To address this problem, we investigated a cross-seeding approach with a mixture integrating a heterogeneous set of protein crystal fragments to be used as generic seeds. The fragments are nanometre-sized templates chosen to promote crystal nucleation of protein samples unrelated to the proteins forming the seeds. To demonstrate applicability, the generic cross-seeding mixture was simply added to a sample of the human retinoblastoma binding protein 9 (RBBP9) before proceeding with crystallization.

An atypical crystal form of the human serine hydrolase retinoblastoma binding protein 9 was obtained by adding the mixture to the protein sample before performing standard crystallization assays. The structure was solved by X-ray crystallography at 1.4 Å resolution. Follow-up experiments showed that crystal fragments of α-amylase were critical components in this particular result. A different crystal morphology was only observed when the seeding mixture was added to the sample in two screening conditions: MORPHEUS-FUSION D5 {12.5% w/v PEG 1000, 12.5% w/v PEG 3350, 12.5% v/v MPD [(RS)-2-methyl-2,4-pentanediol], 0.1 M MOPS/HEPES-Na [4-(2-hydroxyethyl)piperazine-1-ethanesulfonic acid], sodium salt pH 7.5, 20 mM amino acids, 20 mM monosaccharides} and F8 {12.5% w/v PEG 1000, 12.5% w/v PEG 3350, 12.5% v/v MPD, 0.1 M MES [2-(N-morpholino)ethanesulfonic acid]/imidazole pH 6.5, 1 mM alkalis, 0.5% w/v cryo-polyols}. These crystals were single and not elongated [Fig. 3(b)]. However, no unexplained electron density was found that would indicate a cross-seeding fragment caused specific interactions leading to switch the crystal form. However, we could not produce a model describing the possible mechanisms of cross-seeding that could have directly promoted the different crystal form of RBBP9 (space group P212121) with α-amylase fragments, for example by comparing their lattices. In fact, other speculations could be based on indirect effects of the seeds instead of cross-seeding. For example, α-amylase fragments could act as purifying agents, by mobilizing poorly folded RBBP9 molecules, which enabled the growth of a different crystal form.

>MASPSKAVIVPGNGGGDVTTHGWYGWVKKELEKIPGFQCLAKNMPDPITARESIWLPFMETELHCDEKTIIIGHSSGAIAAMRYAETHRVYAIVLVSAYTSDLGDENERASGYFTRPWQWEKIKANCPYIVQFGSTDDPFLPWKEQQEVADRLETKLHKFTDCGHFQNTEFHELITVVKSLLKVPA[2x]> 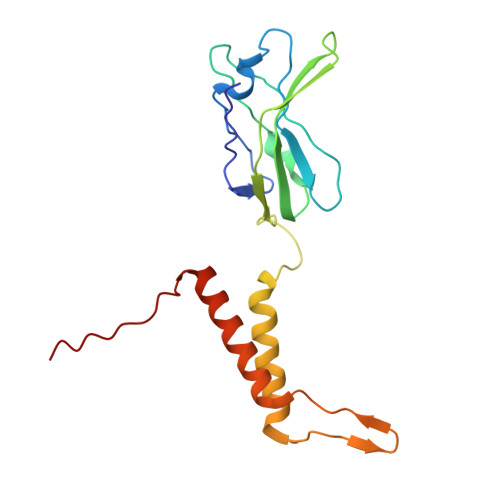MTVSIHPPATLVAGDSWAWEAGAVFEDHPDPWAASYVLRPEAGGDPVTVSGGLEVLAPVFRLPASVTADLPPGEWTWFAVAVDATTDARAVLAQGRVTVIPDPLAGTEDRRTPARRILAAIEATLEGRATKDADTYSIEGRSITRTPLPDLLRLRAVYAEQVARETGRSPYRQRRVSF> MAHHHHHHVDDDDKDLFNKNKKLDADLLKTLDNLLKTLDNNQKQALIYFKDKLQDKKYLNDLMEQQKSFLDNLQKKKEDPDLQDRLKKTLNSEYDESQFNKLLNELGNAKAKQFLQQLHIMLQSIKDGTLTSFSSSNFNDLQNLEQKKERALQYINGKLYVEYYFYIN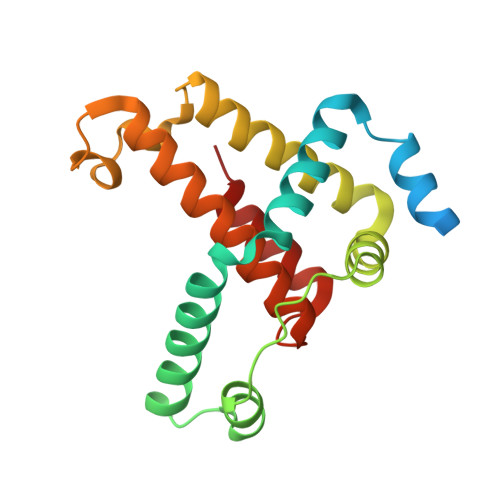GISNADNFFETIMEYLKT>[2x]AKKTPPVYPVTVPFLGHIVQFGKNPLEFMQRCKRD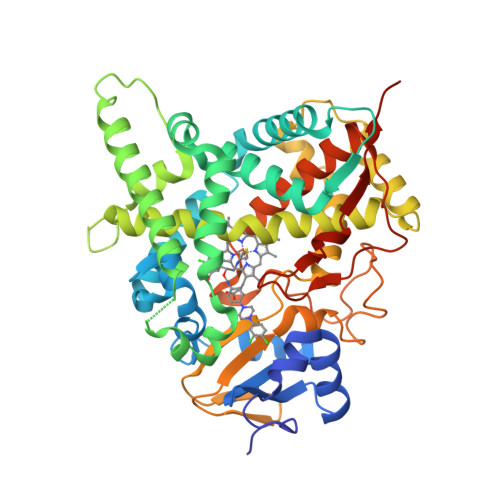LKSGVFTISIGGQRVTIVGDPHEHSRFFSPRNEILSPREVYTIMTPVFGEGVAYAAPYPRMREQLNFLAEELTIAKFQNFVPAIQHEVRKFMAENWKEDEGVINLLEDCGAMIINTACQCLFGEDLRKRLNARHFAQLLSKMESSLIPAAVFMPWLLRLPLPQSARCREARAELQKILGEIIVAREKEEASKDNNTSDLLGGLLKAVYRDGTRMSLHEVCGMIVAAMFAGQHTSTITTSWSMLHLMHPKNKKWLDKLHKEIDEFPAQLNYDNVMDEMPFAERCVRESIRRDPPLLMVMRMVKAEVKVGSYVVPKGDIIACSPLLSHHDEEAFPNPRLWDPERDEKVDGAFIGFGAGVHKCIGQKFALLQVKTILATAFREYDFQLLRDEVPDPDYHTMVVGPTLNQCLVKYTRKKKLPSHHHHHH>[2x]SMLNSELNTKIVNRGKEFFGSISGEKPSLF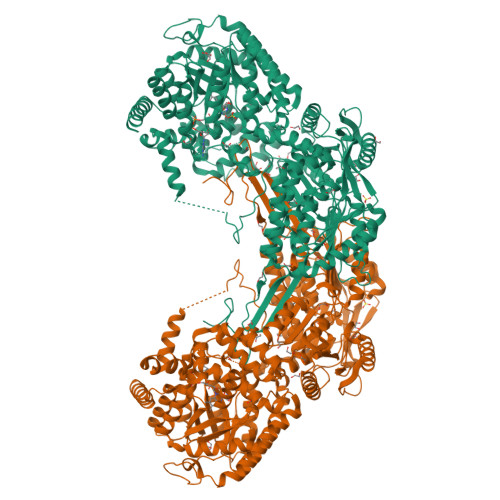NKGAWMGKAMDWSMQNEQFKIQMFRFVDVFPSLTTSKLLTEHIREYFGNEQDMPAFMSTGAKVAGMLGSFGGAVLNKVLTSNIEEMARQFIVGETTKEAVKNLEKLRKDGFAAVVDVLGEATLSEEEAEVYTNTYLELLEALKKEQGSWKGLPGKGGDPGLDWGHAPKVNIAVKPTWLFCLANPQDFEGSVVAILDRMRRIFKKVMELNGFLCIDMESYRHKEIILEVFRRLKLEYRDYPHLGIVLQAYLKDNDKDLDDLLAWAKEHKVQISVRLVKGAYWDYETVKAKQNDWEVPVWTIKAESDAAYERQARKILENHQICHFACASHNIRTISAVMEMARELNVPEDRYEFQVLYGMAEPVRKGILKVAGRIRLYAPYGNMVPGMGYLVRRLLENTANESFLRQSFAEDAQIERLLEDPAVTVERERAARAAKPKKERKGLGGLPPFNNEAMVDFTRADHRAAFPKHIAQVRTQLGKTYPLFINGKEVRTNDLIPTVNPNKPSEVLGQICQAGTTEVGDAIAAAKAAFPAWRDTDPRTRAEYLLKAAQAARKRLFELSAWQVLEIGKQWDQAYADVTEAIDFLEYYAREMIRLGQPQRVGHAPGELNHYFYEPKGVAAVIAPWNFPLAISMGMASAAIVTGNCVVFKPSGITSIIGWHLVELFREAGLPEGVFNFTPGRGSVMGDYLVDHPDISLIAFTGSMETGLRIIERAAKVHPGQANVKKIISEMGGKNAIIIDDDADLDEAVPHVLYSAFGFQGQKCSACSRVIVLDAVYDKFIERLVSMAKATKVGPSEDPANYMGAVADDKAMKSIKEYAEIGKREGHVLYESPVPAGEGYFVPMTIIGGIKPEHRIAQEEIFGPVLAVMRAKDFDQAIEWANSTQFALTGGIFSRSPEHLAKARREFRVGNLYINRNNTGALVERQPFGGARMSGVGTKAGGPDYLLHFMDPRVVTENTMRRGFAPIEEDDDWVD> LPALPEDGGSGAFPPGHFKDPKRLYCKNGGFFLRIHPDGRVDGVREKSDPHIKL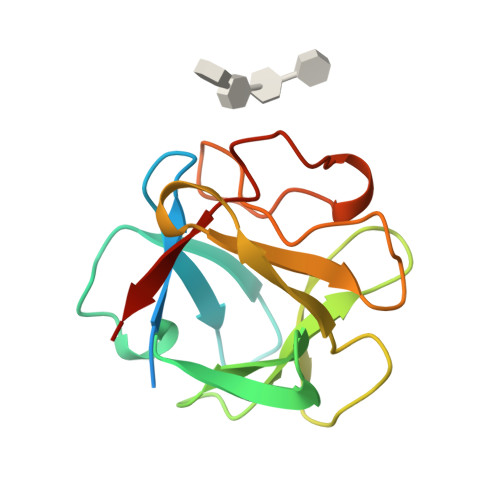QLQAEERGVVSIKGVSANRYLAMKEDGRLLASKSVTDECFFFERLESNNYNTYRSRKYTSWYVALKRTGQYKLGSKTGPGQKAILFLPMSAKS> MDSTKEKCDSYKDDLLLRMGLNDNKAGMEGLDKEKINKIIMEATKGSRFYGNELKKEKQVNQRIENMMQQKAQITSQQLRKAQLQVDRFAMELEQSRNLSNTIVHIDMDAFYAAVEMRDNPELKDKPIAVGSMSMLSTSNYHARRFGVRAAMPGFIAKRLCPQLIIVPPNFDKYRAVSKEVKEILADYDPNFMAMSLDEAYLNITKHLEERQNWPEDKRRYFIKMGSSVENDNPGKEVNKLSEHERSISPLLFEESPSDVQPPGDPFQVNFEEQNNPQILQNSVVFGTSAQEVVKEIRFRIEQKTTLTASAGIAPNTMLAKVCSDKNKPNGQYQILPNRQAVMDFIKDLPIRKVSGIGKVTEKMLKALGIITCTELYQQRALLSLLFSETSWHYFLHISLGLGSTHLTRDGERKSMSVERTFSEINKAEEQYSLCQELCSELAQDLQKERLKGRTVTIKLKNVNFEVKTRASTVSSVVSTAEEIFAIAKELLKTEIDADFPHPLRLRLMGVRISSFPNEEDRKHQQRSIIGFLQAGNQALSATECTLEKTDKDKFVKPLEMSHKKSFFDKKRSERKWSHQDTFKCEAVNKQSFQTSQPFQVLKKKMNENLEISENSDDCQILTCPVCFRAQGCISLEALNKHVDECLDGPSISENFKMFSCSHVSATKVNKKENVPASSLCEKQDYEAHPKIKEISSVDCIALVDTIDNSSKAESIDALSNKHSKEECSSLPSKSFNIEHCHQNSSSTVSLENEDVGSFRQEYRQPYLCEVK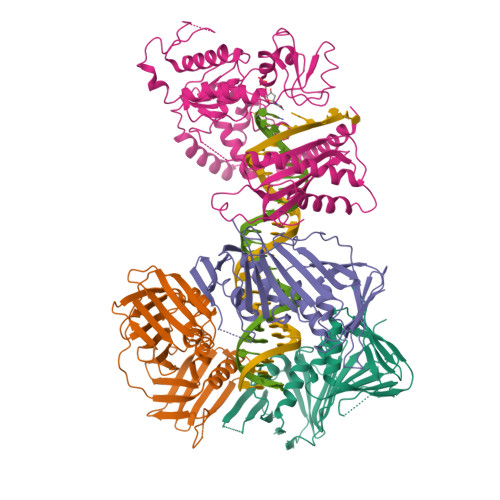TGQALVCPVCNVEQKTSDLTLFNVHVDVCLNKSFIQELRKDKFNPVNQPKESSRSTGSSSGVQKAVTRTKRPGLMTKYSTSKKIKPNNPKHTLDIFFK;>[3x]GPHMFEARLVQGSILKKVLEALKDLINEACWDISSSGVNLQSMDSSHVSLVQLTLRSEGFDTYRCDRNLAMGVNLTSMSKILKCAGNEDIITLRAEDNADTLALVFEAPNQEKVSDYEMKLMDLDVEQLGIPEQEYSCVVKMPSGEFARICRDLSHIGDAVVISCAKDGVKFSASGELGNGNIKLSQTSNVDKEEEAVTIEMNEPVQLTFALRYLNFFTKATPLSSTVTLSMSADVPLVVEYKIADMGHLKYYLAPKIEDEEGS> GAKPYEKVRIYRMDGS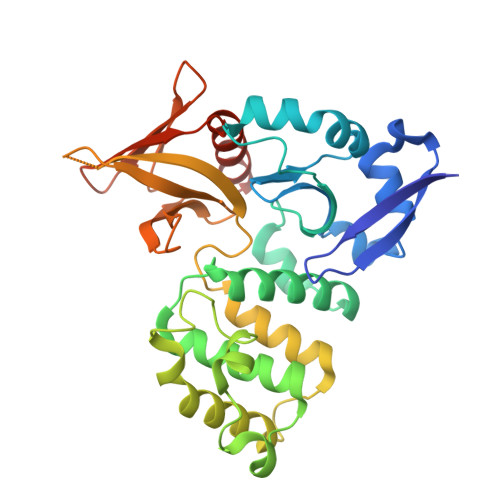YRSVELKHGNNTTVQQIMEGMRLSQETQQYFTIWICSENLSLQLKPYHKPLQHVRDWPEILAELTNLDPQRETPQLFLRRDVRLPLEVEKQIEDPLAILILFDEARYNLLKGFYTAPDAKLITLASLLLQIVYGNYESKKHKQGFLNEENLKSIVPVTKLKSKAPHWTNRILHEYKNLSTSEGVSKEMHHLQRMFLQNCWEIPTYGAAFFTGQIFTKASPSNHKVIPVYVGVNIKGLHLLNMETKALLISLKYGCFMWQLGDTDTCFQIHSMENKMSFIVHTKQAGLVVKLLMKLNGQLMPTERNS> GPLGSPRYELGEELRDKIKQEPSFSNMVSAKKFYNKAIKDFTAPKEGAEVVSVKTHIMRPIDFMLM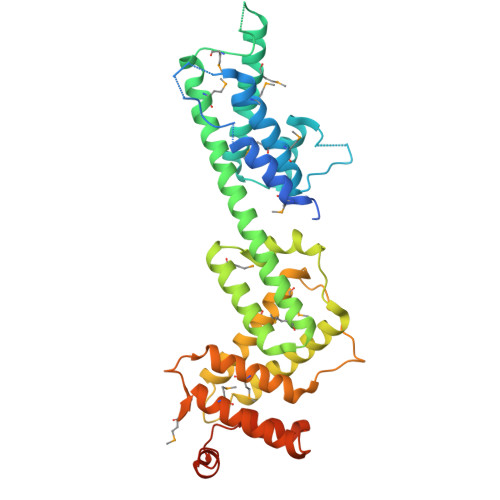GLREEFNLYSEDGAHLSAPGTIRLLREKNLLPEEQIARIESVYNQAMSKRFELHAEHKKEHDEMPYSDAKAMLDEVAKIRELGVQRVTRIENLENAKKLWDNANSMLEKGNISGYLKAANELHKFMKEKNLKEDDLRPELSDKTISPKGYAILQSLWGAASDYSRAAATLTESTVEPGLVSAVNKMSAFFMDCKLSPNERATPDPDFKVGKSKILVGIMQFIKDVADPTSKIWMHNTKALMNHKIAAIQKLERSNNVNDETLESVLSSKGENLSEYLSYKYATKDEGREHRYTASTE> TYKATHEFMSGTPGKELPQEVKDLLPADQTDLKDGSQATPTQPSKTEVKTAEGTWSFKSYDKTSETINGADAHFVGTWEFTPAPTYKATHEFVSGTPGKELPQE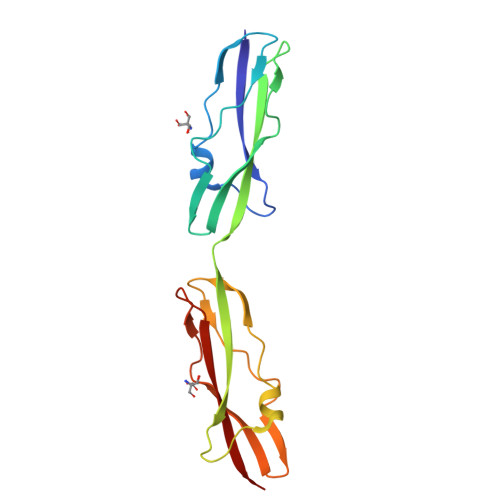VKDLLPADQTDLKDGSQATPTQPSKTEVKTTEGTWSFKSYDKTSETINGADAHFVGTWEFTPA> MQIVVLAKVVPDYEVPSADFELVGNRAHPRYTRMIGLYDENAVELGVQLKEKLGADLTVVSYGRNDDVQFLRKALAMGADKVVLVEGDSDDPYVIAANLKDAIDRQGTVDLILAGRQSSDMD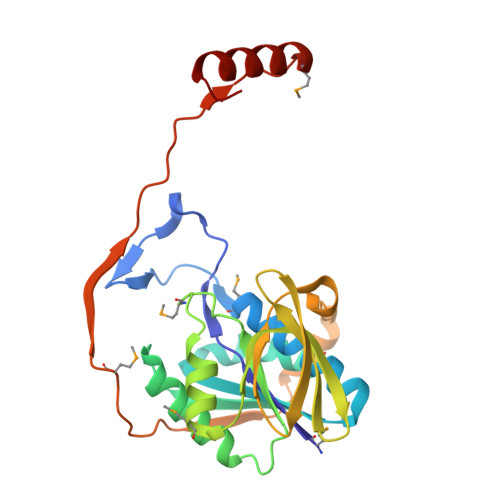RGVVPGVLAGMLDLPFVPQACSVESVDGGWKISQITETGKRLLKLSGKGVLSITSVPENVPRIPAVKAIFAAKKKPVEKLPEIGTGKMAVSELSVSIPKVESNCELIPAEDMDDAVRVLLRRLKEERYL>MGHMNITDIREQFPILHQQVNGHDLVYLDSAATSQKPRAVIETLDKYYNQYNSNVHRGVHTLGTRATDGYEGAREKVRKFINAKSMAEIIFTKGTTTSLNMVALSYARANLKPGDEVVITYMEHHANIIPWQQAVKATGATLKYIPLQEDGTISLEDVRETVTSNTKIVAVSHVSNVLGTVNPIKEMAKIAHDNGAVIVVDGAQSTPHMKIDVQDLDCDFFALSSHKMCGPTGVGVLYGKKALLENMEPAEFGGEMIDFVGLYESTWKELPWKFEAGTPIIAGAIGLGAAIDFLEEIGLDEISRHEHKLAAYALERFRQLDGVTVYGPEERAGLVTFNLDDVHPHDVATVLDAEGIAVRAGHHCAQPLMKWLDVTATARASFYLYNTEEEIDKLVEALQKTKEYFTNVFVDLEHHHHHH[2x];>MSFNANLDTLYRQVIMDHYKNPRNKGVLNDSIVVDMNNPTCGDRIRLTMKLDGDIVEDAKFEGEGCSISM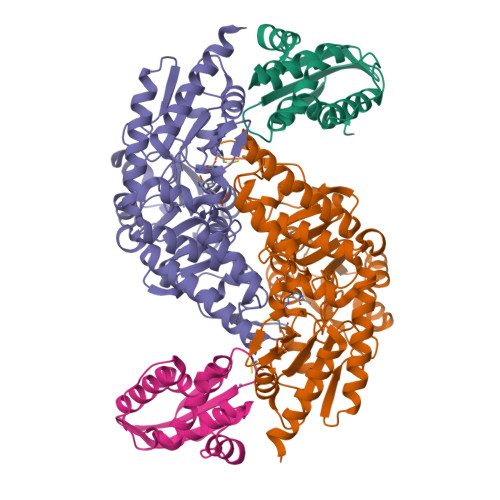ASASMMTQAIKGKDIETALSMSKIFSDMMQGKEYDDSIDLGDIEALQGVSKFPARIKCATLSWKALEKGVAKEEGGNLEHHHHHH[2x]> GPGSMVDGSDGARRVLVINSGSSSLKFQLVDPESGVAASTGIVERIGEESSPVPDHDAALRRAFDMLAGDGVDLNTAGLVAVGHRVVHGGNTFYRPTVLDDAVIARLHELSELAPLHNPPALLGIEVARRLLPGIAHVAVFDTGFFHDLPPAAATYAIDRELADRWQIRRY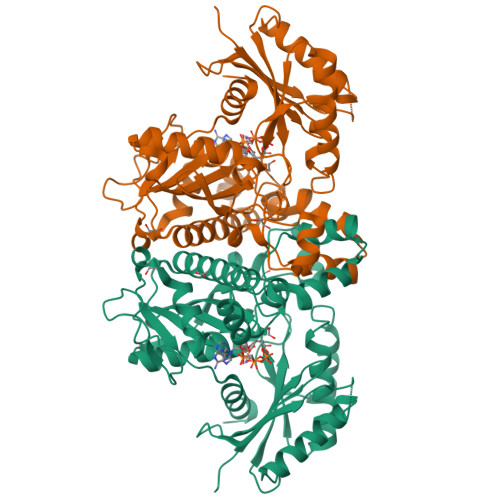GFHGTSHRYVSEQAAAFLDRPLRGLKQIVLHLGNGCSASAIAGTRPLDTSMGLTPLEGLVMGTRSGDIDPSVVSYLCHTAGMGVDDVESMLNHRSGVVGLSGVRDFRRLRELIESGDGAAQLAYSVFTHRLRKYIGAYLAVLGHTDVISFTAGIGENDAAVRRDAVSGMEELGIVLDERRNLPGAKGARQISADDSPITVLVVPTNEELAIARDCVRVLGG>[2x]MASSLKQGVSPKLRDVILVSKDIPEQLCDALFFYTSHNPKDYADAFAVRQKFDRNLQTGKQFKFETVCGLFLLKGVDKITPGVPAKVLKATSKLADLEDIFGVSPFARKYRELLKTACQWSLTVEALDVRAQTLDEIFDPTEILWLQVAAKIHVSSMAMRRLVGEVTAKVMDALGSNLSALFQIFKQQIVRIFQKALAIFENVSELPQRIAALKMAFAKCARSITVVVMERTLVVREFAGTCLASINGAVAKFFEELPNGFMGAKIFTTLAFFKEAAVRIVENIPNAPRGTKGFEVVGNAKGTQVVVRGMRNDLTLLDQKADIPVESEGWSAILGGHLCYVFRSGDRFYAAPLSGNFALHDVHCCERVVCLSDGVTPEINDGLILAAIYSSFSVAELVAAIKKGEPFKFLGHKFVYAKDAAVSFTLAKAATIADVLRLFQSARVKVEDVWSSLTEKSFEFWRLAYGKVRNLEEFVKTCFCKAQMAIVI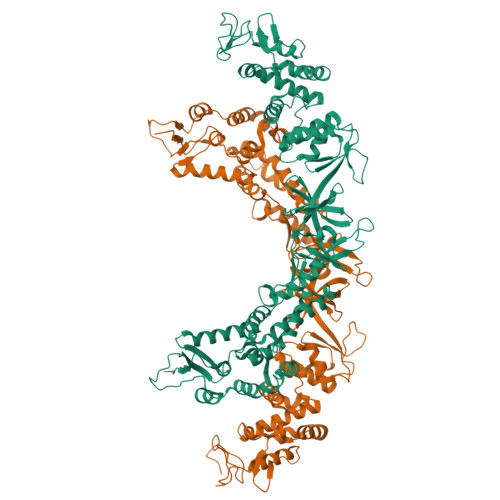LATVLGEGIWHLVSQVIYKVGGLFTKVVDFCEKYWKGFCAQLKRAKLIVTETLCVLKGVAQHCFQLLLDAIQFMYKSFRKCALGRIHGDLLFWKGGVHKIIQEGDEIWFDAIDSVDVEDLGVVQEKSIDFEVCDDVTLPENQPGHMVQIEDDGKNYMFFRFKKDENIYYTPMSQLGAINVVCKAG>TCRYLLVRSLQTFSQAWFTCRRCYRGNLVSIHNFNINYRIQCSVSALNQGQVWIGGRITGSGRCRRFQWVDGSRWNFAYWAAHQPWSRGGHCVALCTRGGYWRRAHCLRRLPFICS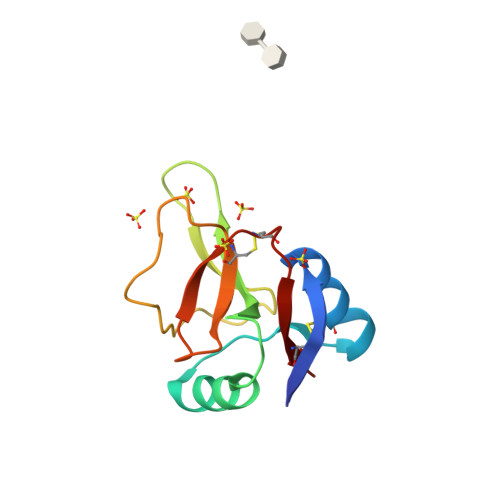Y[2x]>GSHGMRVIIAGFGRFGQITGRLLLSSGVKMVVLDHDPDHIETLRKFGMKVFYGDATRMDLLESAGAAKAEVLINAIDDPQTNLQLTEMVKEHFPHLQIIARARDVDHYIRLRQAGVEKPERETFEGALKTGRLALESLGLGPYEARERADVFRRFNIQMVEEMAMVENDTKARAAVYKRTSAMLSEIITEDREHLSLIQRHGWQGTEEGKHTGNMADEPETKPSSTSGGLVPRGSSGMILIIYAHPYPHHSHANKRMLEQARTLEGVEIRSLYQLYPDFNIDIAAEQEALSRADLIVWQHPMQWYSIPPLLKLWIDKVFSHGWAYGHGGTALHGKHLLWAVTTGGGESHFEIGAHPGFDVLSQPLQATAIYCGLNWLPPFAMHCTFICDDETLEGQARHYKQRLLEWQEAHHG[2x]

KTN (RCK) domains are nucleotide-binding folds that form the cytoplasmic regulatory complexes of various K+ channels and transporters. Many of these proteins, including E. coli KefC and KefB, are glutathione (GSH)-gated K+ efflux systems that are usually maintained in a closed state. Exposure of the cell to electrophiles leads to the formation of GSH adducts (GSX) that are activators of the efflux system (Elmore et al., 1990; Ferguson et al., 1995). KefF is essential for full activation of the KefC system and therefore appears to be an integral part of the system's gating machinery.

In this report, we present the structure of the KTN-bearing C-terminal domain of E. coli KefC (KefC-CTD) in complex with KefF, resolved to 2.4 Å resolution. In order to stabilize the KefC-CTD/KefF complex for structural analysis, fusion of the two domains via a flexible 12-residue synthetic linker was pursued. Crystals contain one dimer of the fusion complex within the asymmetric unit. Although all of the residues of KefF could be constructed from the resulting electron density maps, much of the C-terminal peripheral domain of KefC-CTD, as well as all of the artificial linker, are disordered. The structure reveals that KefF binds to the ends of the hinge-forming arms of KefC's KTN domain, fixing this hinge at approximately 120°. Unexpectedly, the structure reveals that KefF has a novel zinc binding site not found in the other quinone reductase enzymes with which it shares homology. The metal cation is bound primarily by three KefF residues: H12, H13, and Q37. Further, this zinc forms part of the extensive interface between the two subunits of the Kef system, being also coordinated by a backbone amide group belonging to G536 of KefC. The cofactor for this protein was determined to be FMN by mass spectroscopy, a conclusion that is consistent with the observed electron density in the structure. A binding pocket for GSH between this arm and the rest of the KTN domain suggests that the arm can either be stabilized in the obstructive conformation by a smaller GSH molecule or possibly destabilized by bulkier GSH adducts, modifying in turn the protein interaction interface's potential ability to associate with parts of the membrane domain, which might lead to activation of K+ efflux.> MEGSTGFDGDATTFFAPDAVFGDRVRRFQEFLDTFTSYRDSVRSIQVYNSNNAANYNDDQDDADERDLLGDDDGDDLEKEKKAASSTSLNILPHRIIISLDDLREFDRSFWSGILVEPAYFIPPAEKALTDLADSMDDVPHPNASAVSSRHPWKLSFKGSFGAHALSPRTLTAQHLNKLVSVEGIVTKTSLVRPKLIRSVHYAAKTGRFHYRDYTDATTTLTTRIPTPAIYPTEDTEGNKLTTEYGYSTFIDHQRITVQEMPEMAPAGQLPRSIDVILDDDLVDKTKPGDRVNVVGVFKSLGAGGMNQSNSNTLIGFKTLILGNTVYPLHARSTGVAARQMLTDFDIRNINKLSKKKDIFDILSQSLAPSIYGHDHIKKAILLMLMGGVEKNLENGSHLRGDINILMVGDPSTAKSQLLRFVLNTASLAIATTGRGSSGVGLTAAVTTDRETGERRLEAGAMVLADRGVVCIDEFDKMTDVDRVAIHEVMEQQTVTIAKAGIHTTLNARCSVIAAANPVFGQYDVNRDPHQNIALPDS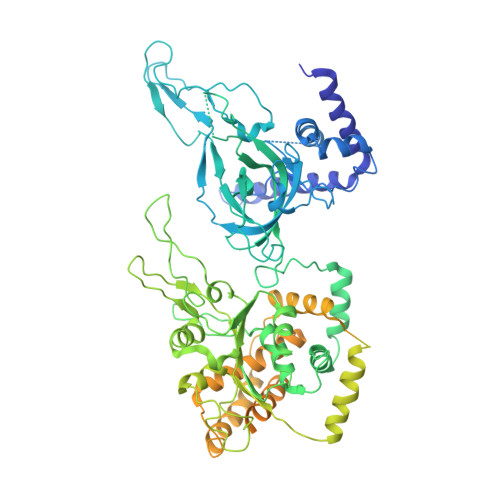LLSRFDLLFVVTDDINEIRDRSISEHVLRTHRYLPPGYLEGEPVRERLNLSLAVGEDADINPEEHSNSGAGVENEGEDDEDHVFEKFNPLLQAGAKLAKNKGNYNGTEIPKLVTIPFLRKYVQYAKERVIPQLTQEAINVIVKNYTDLRNDDNTKKSPITARTLETLIRLATAHAKVRLSKTVNKVDAKVAANLLRFALLGEDIGNDIDEEESEYEEALSKRSPQKSPKKRQRVRQPASNSGSPIKSTPRRSTASSVNATPSSARRILRFQDDEQNAGEDDNDIMSPLPADEEAELQRRLQLGLRVSPRRREHLHAPEEGSSGPLTEVGTPRLPNVSSAGQDDEQQQSVISFDNVEPGTISTGRLSLISGIIARLMQTEIFEEESYPVASLFERINEELPEEEKFSAQEYLAGLKIMSDRNNLMVADDKVWRV2-(1-{[2-(2-aminopyrimidin-5-yl)-4-(morpholin-4-yl)pyrido[3,2-d]pyrimidin-6-yl]methyl}piperidin-4-yl)propan-2-ol | C24 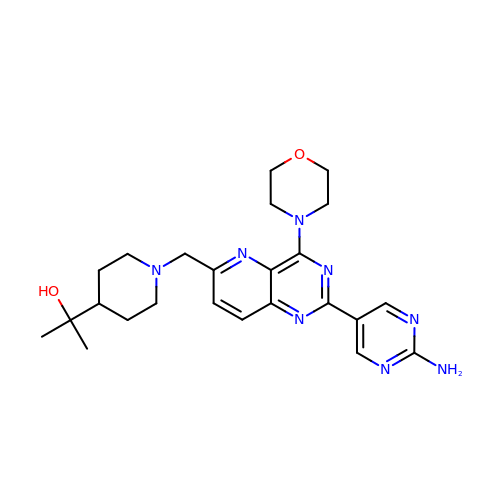H32 N8 O2 | SQGDUMWGWUGDIS-UHFFFAOYSA-N> GLGDLIEGVVEGVTRNALTPLTPANNLPDTQSSGPAHSKETPALTAVETGATNPLVPSDTVQTRHVIQKRTRSESTVESFFARGACVAIIEVDNDAPTKRASKLFSVWKITYKDTVQLRRKLEFFTYSRFDMEFTFVVTSNYTDANNGHALNQVYQIMYIPPGAPIPGKWNDYTWQTSSNPSVFYTYGAPPARISVPYVGIANAYSHFYDGFAKVPLA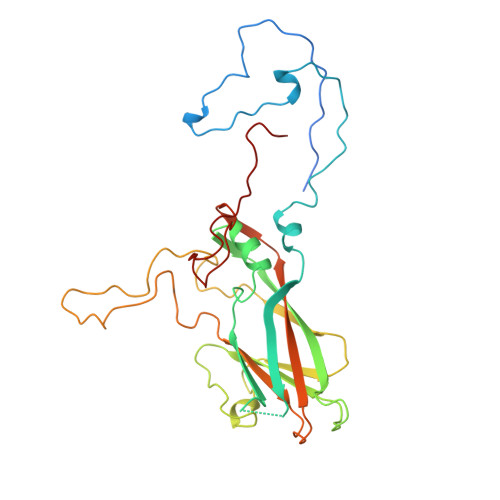GQASTEGDSLYGAASLNDFGSLAVRVVNDHNPTKLTSKIRVYMKPKHVRVWCPRPPRAVPYYGPGVDYKDGLAPLPGKGLTTY>[6x]MQLTRLVQVDCPLGPDVLLLQRMEGREELGRLFAYELHLVSENPNLPLEQLLGKPMSLSLELPGGSRRFFHGIVARCSQVAGHGQFAGYQATLRP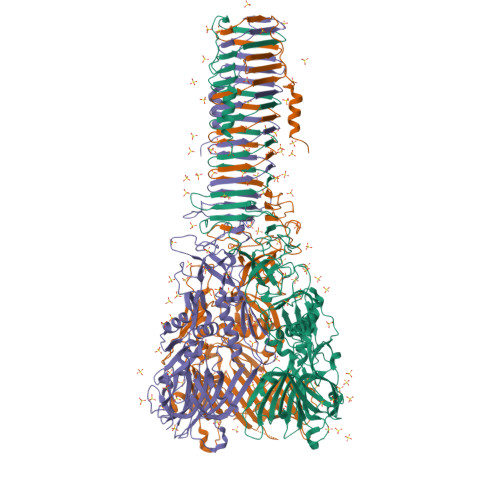WPWLLTRTSDCRIFQNQSVPEIIKQVFRNLGFSDFEDALTRPYREWEYCVQYRETSFDFISRLMEQEGIYYWFRHEQKRHILVLSDAYGAHRSPGGYASVPYYPPTLGHRERDHFFDWQMAREVQPGSLTLNDYDFQRPGARLEVRSNIARPHAAADYPLYDYPGEYVQSQDGEQYARNRIEAIQAQHERVRLRGVVRGIGAGHLFRLSGYPRDDQNREYLVVGAEYRVVQELYETGSGGAGSQFESELDCIDASQSFRLLPQTPVPVVRGPQTAVVVGPKGEEIWTDQYGRVKVHFHWDRHDQSNENSSCWIRVSQAWAGKNWGSMQIPRIGQEVIVSFLEGDPDRPIITGRVYNAEQTVPYELPANATQSGMKSRSSKGGTPANFNEIRMEDKKGAEQLYIHAERNQDNLVENDASLSVGHDRNKSIGHDELARIGNNRTRAVKLNDTLLVGGAKSDSVTGTYLIEAGAQIRLVCGKSVVEFNADGTINISGSAFNLYASGNGNIDTGGRLDLNSGGASEVDAKGKGVQGTIDGQVQAMFPPPAKG>LESPGFMVHKKLKSMSQSYGVMMTGVPAEVLGQMQAERSIPSINKTGNLKQQIAKEVSKVCHMMTEPTQSCGQASNDVCELLLGKIEAEKFHFTKYEALSADGDNLKNVLENTAPSSTNLLIRFEIDREDPPIVLVKTKNENFNPETAVKNKIYLLENKLYFIDKMGNLFNLGPGKKKCTQLFNAIGDSAEYSLCDPFVLEEPEKPEDFAISEIVDIFNEQKERFDFWIGSHSFTIYIPQTLGESPRQFYPYQAYFGSHTLQDWFVSDKDEYLSRIGIDKYIEKLAVLGKTTNTKERSDIYAEFFSKRGREAFFCAHLNEKRQPLRVKFKITEINPELAL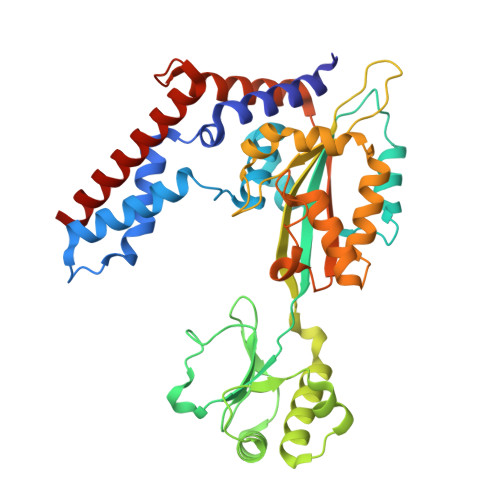KNLQETQEFIDTHPGENPSDKVENYRNRAKLAMTEHLESLLDI[2x]> MPVLNLNDPQAVERYEEFMRQSPYGQVTQDLGWAKVKNNWEPVDVYLEDDQGAIIAAMSMLLGDTPTDKKFAYASKGPVMDVTDVDLLDRLVDEAVKALDGRAYVLRFDPEVAYSDEFNTTLQDHGYVTRNRNVADAGMHATIQPRLNMVLDLTKFPDAKTTLDLYPSKTKSKIKRPFRDGVEVHSGNSATELDEFFKTYTTMAERHGITHRPIEYFQRMQAAFDADTMRIFVAEREGKLLSTGIALKYGRKIWYMYAGSMDGNTYYAPYAVQSEMIQW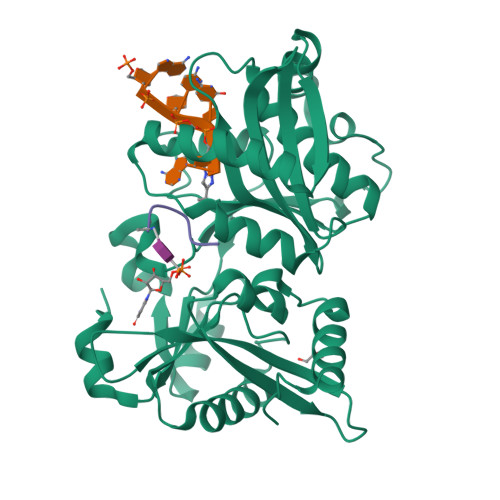ALDTNTDLYDLGGIESESTDDSLYVFKHVFVKDAPREYIGEIDKVLDPEVYAELVKDGHHHHHH;> AECAA>MDPEVFAQARLRMDQLTKPPRALGYLEEVALRLAALQGRVKPELGRGAVVVAAADHGVVAEGVSAYPQEVTRQMVLNFLRGGAAINQFALAADCAVYVLDVGVVGELPDHPGLLKRKVRPGTANLAQGPAMTPEEAERALLAGREAARRAIAEGATLLAAGDMGIGNTTAAAALTAALLGLPPEAVVGRGTGVGEEGLRRKRQAVARALARLHPGMGPLEVAAEVGGLELV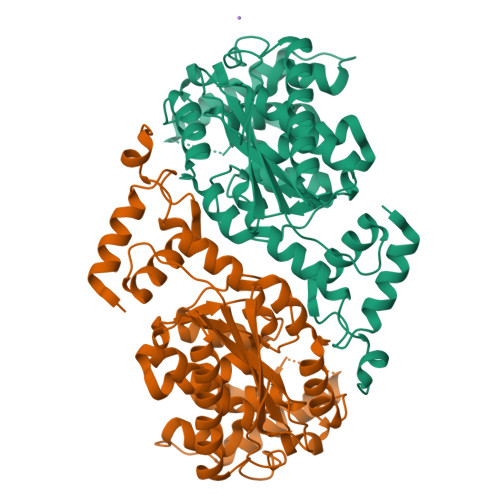AIAGIYLEGYEAGLPLVLDGFPVTAGALLAWKMAPGLRDHLFAGHLSREPGHRHQLEALGLRPLLDLDLALGEGTGAVLAMPLLRAAARILHMATFQEAGVSRG[2x]> GPAFSKKVLGSNPSSGKEVALTFDDGPFPIYTEKYVDILKSMDVKATFFVIGKHAEKHPELLKYIVENGNEIGLHSYSHFNMKKLKPEKMVEELYKTQQIIVEATGIKPTLFRPPFGAYNSTLIEISNALGLKVVLWNVDPDDWRNPSVESVVNRVLSHTRDGSIILMHEGKPSTLAALPQIIKKLKEEGYKFVTVSELL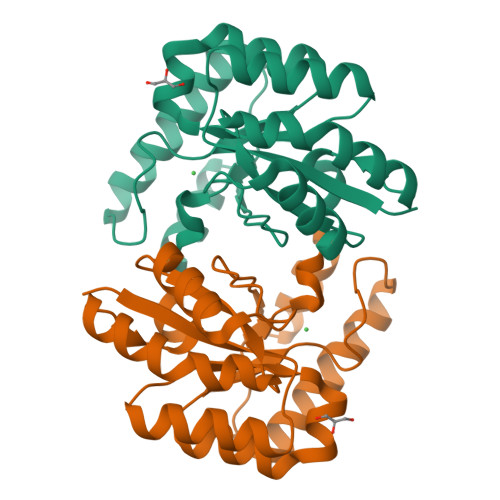EKRD> MTTQQPEWTQAASDLMARTAALARKKANGYLDPVHLAYVMFEDENSLASRVVRKLGAASVKDGLEARVDAIPTQMPAPTQPRPNSDMMRVMNTAEQERVALGDTLMAADHFLLALHESKEV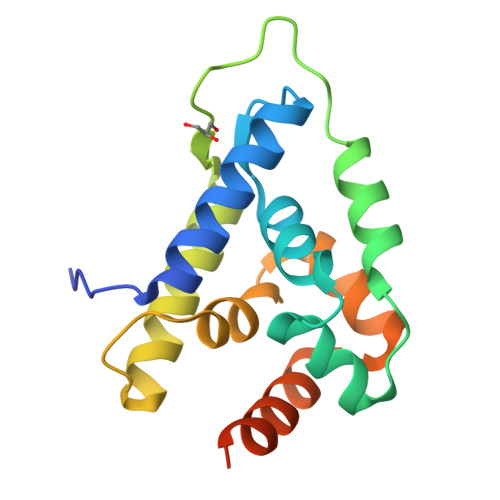GRILDAAGAGKKAIRTTLLEMRKGKKITSDFQDDNYE>APTENSTGVQDCYRGDGQSYRGTLSTTITGRTCQSWSSMTPHWHRRIPLYYPNAGLTRNYCRNPDAEIRPWCYTMDPSVRW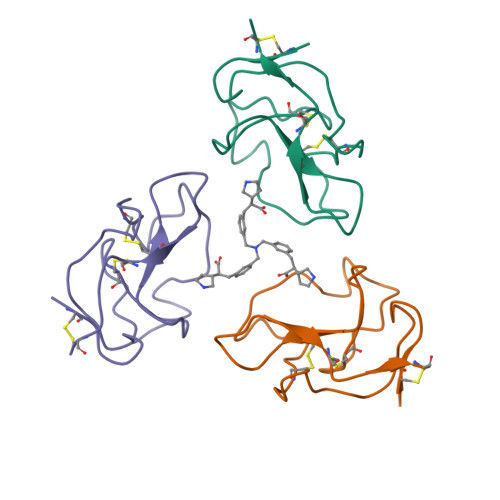EYCNLTRCPVTES[3x]>AAVLQQVLERTELNKLPKSVQNKLEKFLADQQSEIDGLKGRHEKFKVESEQQYMEIEKRLSHSQERLVNETRECQSLRLELEKLNNQLKALTEKNKELEMAQDRNIAIQSQMTRT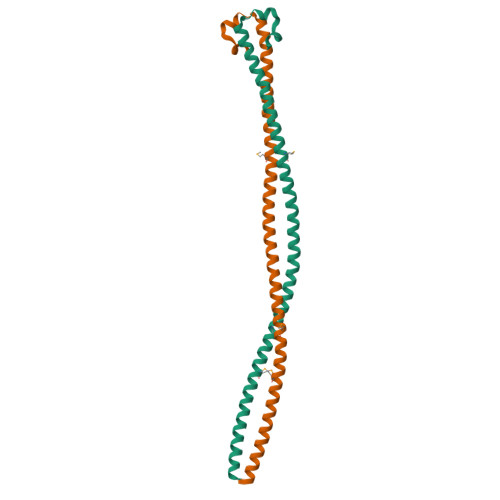KEELEAEKRDLIRTNERLSQELEYLT[2x]During bacterial cell division, filaments of tubulin-like FtsZ form the Z-ring, which is the cytoplasmic scaffold for divisome assembly. In Escherichia coli, actin homologue FtsA anchors the Z-ring to the membrane and recruits divisome components, including bitopic FtsN. In E. coli and many other bacteria, FtsA is the main membrane anchor for the cell division ring, the Z-ring, which initiates and organises division.

The EcFtsA1-405 and XpFtsA1-396 structures showed single protofilaments with a “loose” longitudinal contact between the IIA and IIB subdomains. We noticed that the position of the IC domain is variable within FtsA monomers across FtsA structures.

> MIKATDRKLVVGLEIGTAKVAALVGEVLPDGMVNIIGVGSCPSRGMDKGGVNDLESVVKCVQRAIDQAELMADCQISSVYLALSGKHISCQNEIGMVPISEEEVTQEDVENVVHTAKSVRVRDEHRVLHVIPQEYAIDYQEGIKNPVGLSGVRMQAKVHLITCHNDMAKNIVKAVERCGLKVDQLIFAGLASSYSVLTEDERELGVCVVDIGGGTMDIAVYTGGALRHTKVIPYAGNVVTSDIAYAFGTPPSDAEAIKVRHGCALGSIVGKDESVEVPSVGGRPPRSLQRQTLAEVIEPRYTELLNLVNEEILQLQEKLRQQGVKHHLAAGIVLTGGAAQIEGLAACAQRVFHTQVRIGAPLNITGLTDYAQEPYYSTAVGLLHYGKESHLNGEAEVEKRVTASV> MNVGDRVRVTSSVVVYHHPEHKKTAFDLQGMEGEVAAVLTEWQGRPISAN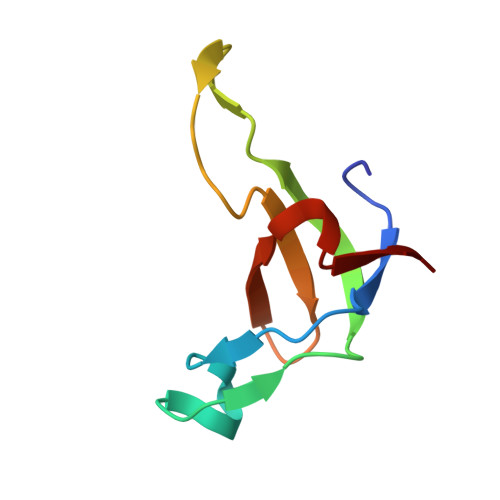LPVLVKFEQRFKAHFRPDEVTLI> EAVTDHPDRLWAWEKFVYLDEKQHAWLPLTIEIKDRLQLRVLLRREDVVLGRPMTPTQIGPS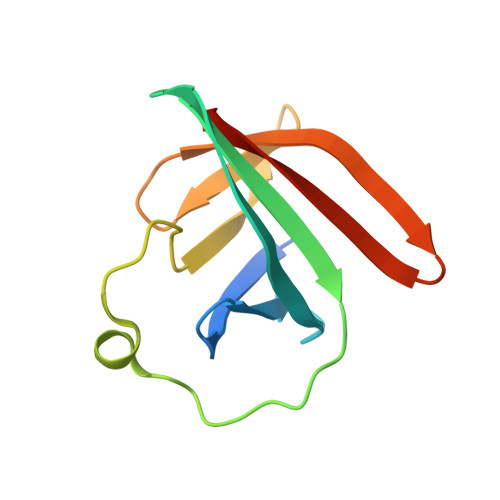LLPIMWQLYPDGRYRSSDSSFWRLVYHIKIDGVEDMLLELLPDD>SNAMADLLLGVNIDHIATLRNARGTIYPDPVQAAFIAEQAGADGITVHLREDRRHITDRDVRILRQTIQTRMNLEMAVTDEMVDIACDIKPHFCCLVPEKRQEVTTEGGLDVAGQVDKMTLAVGRLADVGILVSLFIDADFRQIDAAVAAGAPYIEIHTGAYADASTVLERQAELMRIAKAATYAAGKGLKVNAGHGLTYHNVQPIAALPEMHELNIGHAIIGQAVMTGLAAAV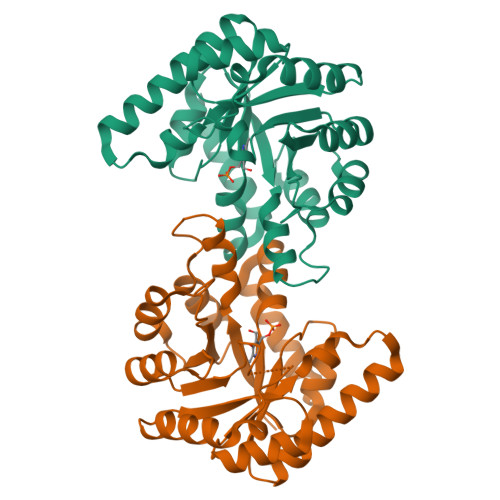TDMKVLMREARR[8x]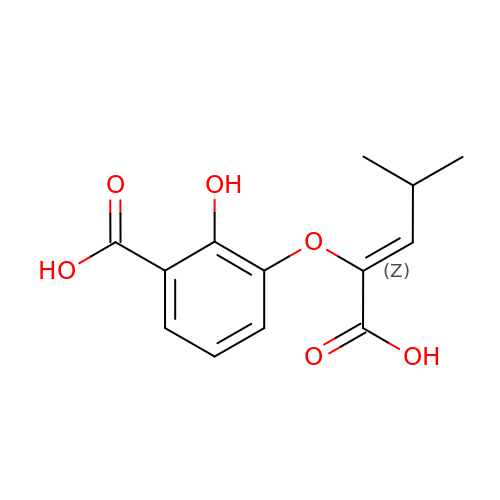3-{[(1Z)-1-carboxy-3-methylbut-1-en-1-yl]oxy}-2-hydroxybenzoic acid | C13 H14 O6 | JVNCGLFIPFSTSG-POHAHGRESA-N>HHHHHHNKDLKGLYAALLVPFDENGQVNEQGLKQIAQNAIETEELDGLYVNGSSGENFLLNTEQKKQVFKVAKEAVGDKVKLIAQVGSLDLNEAIELGKYATELGYDALSAVTPFYYPFTFEEIRDYYFDIIEATQNNMIIYAIPDLTGVNISIEQFSELFNHEKIVGVKYTAPNFFLLERIRKAFPDKLILSGFDEMLVQATISGVDGAIGSTYNVNGRRARKIFDLARQGQIQEAYQLQHDSNDIIETVLSMGIYPTLKEILRHRGIDAGLPKRPFKPFNEAHRQTLDQLIAKYDL[4x]

NAL catalyses the reversible aldol condensation of N-acetylmannosamine with pyruvate to yield the sialic acid, N-acetylneuraminic acid (Neu5Ac). NAL is a class I aldolase, functioning through the formation of an enzyme–pyruvate Schiff base formed with Lys165 which carries out a nucleophilic attack on the aldehyde carbon of the open-chain form of the N-acetylmannosamine. Here, using the NAL from Staphylococcus aureus, we demonstrate quantitative conversion of a cysteine residue, site-specifically into the nonproteogenic amino acid γ-thialysine, chosen as a mimic of the natural catalytic lysine residue at position 165, using the double alkylation-elimination method and that high yields of an active, modified NAL can be purified. We then characterise the resulting enzyme activity, analyse the pH-dependency of catalysis and use X-ray crystallography to investigate the structural basis of the changes brought about by modifying the enzyme.

The effect of Schiff base formation in the S. aureus enzyme is also similar to that found with the E. coli enzyme, namely that it causes ordering of the loop region (138–146) which is not resolved in apo structures. This results in a repositioning of Tyr137, a residue noted as being involved in substrate stabilisation and/or catalysis.> MPPFRQVGEKQLPHEIIFLAWSPKRDLIALVNKAGEVLLHRLANIQRVWSLPPNENTGKEVTCLAWRPDGKILAFGLADTKKVILCDVEKPESLHSFSLETPISCMQWMEVNVENSVLTSFYNAEDEANVLLPKLPALPKNYTATAKIFSEEKSDEILKLLGDARLNALVLGGDSGQIEIYAYGMYKIATISEVYGSCLRLCLSSDLKSLSVVTELTTNNTPEITYFQLDTSLLSDYLPEVTRMARKFTHISTLLQYLQLSLTCMCEAWEEILMQMDSRLTKFVQEKNTTTSVQDEFMQLLLWGKASPELQTLLMNQLTVKGLKKLGQSVESSYSTIQKLVISHLQSGAEALLYHLSELKGMALWRQKYEPLGLDAKAIEDAITAVGSFILKAHELLQVIDSGMKNFKAFFRWLYVAMLRMSEDHVLPELNKMTQKDITFVADFLTEHFNEAPDMYNQKGKYFNVERVGQYLKDEDDILMSPPNIEGNQWFSFLQSSTHLKESPLLFPYYPEKSLHFVKRQMEAIIDR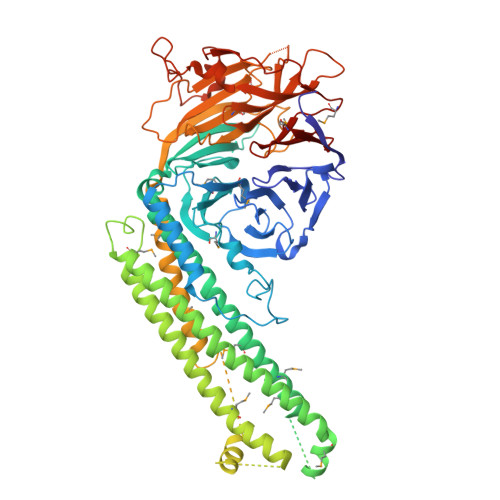CLTKPAQIIGASVQQKRCLPLYQVSASEEACPRLISLPYLWNDKSQNLHCVMFRMLESSSSKVFILRQPTDLSRSINEALLAVTIGNSLNSSAAEDTETSSYSCLDARFYDEDIITVVLRDNSEPEGKDRVLSQLSLSQLYSDEETEDEFTWDTSKRLEEQHSDIPTRTVFLENQGRLLENMKAHYVSVNGIRKVACVLSSNLRHVRVFEMDA>GPTAVQELNRICDGMILSSILRPQMVEPSLIGDVLKTEPFTSSLEVLKDIKVSGLMRYIKQVLLGRKSYYKFGEEHADGDQNLFDYQFTGTPEEPIKGYWTTTISYRDSKPKISLTIRQEFVEGGVESQAVLATVVGRPHLQDFLLLKRKHLEYSDYPESIDLIEFGDVKVIEKTVGHGQPVVLYMASLFPIGLTKIAEQGIGCHNEKNDATLKSLLKTAILNMTPDDVSLLPRSKLDAIDHVVRNVYLRFNNSSAVSYGLHKLQSFEKILQLNGRIYETKESTLVFHHKKGVLVEDLKGLMSYKTLRVS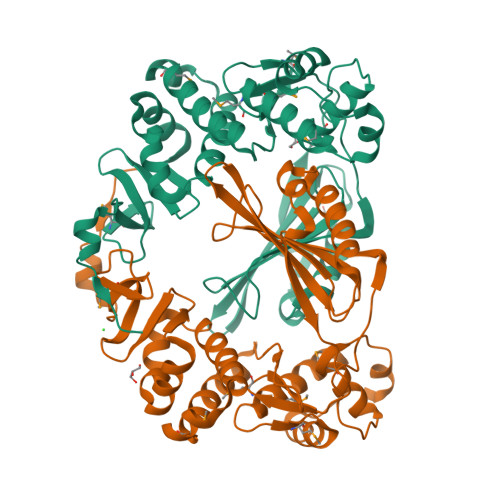EWREKQEPEEARVEVLEE[2x]> GPGSMSETIIEKYADTDALVTAAGDRLASAITGALAERGKAMIVLTGGGTGIALLKHLRDVASGLDWTNVHVFWGDDRYVPKTDPERNAWQAWEALLEHVNFPLRNMHAMPNSESEYGTDL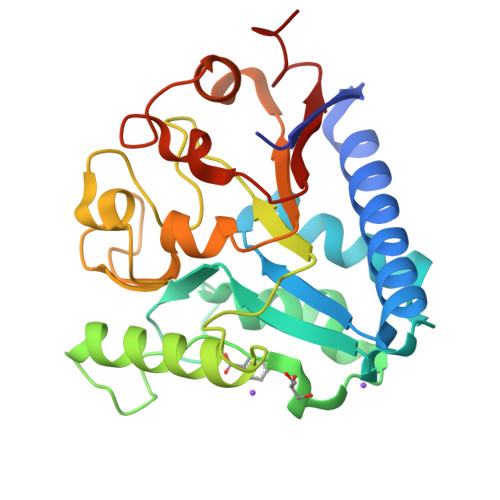DAAALAYEQLLAANAEPGQDCPAFDVHLLGMGGEGHINSLFPHTDAVKETQRLVVAVPDSPKPPPQRITLTLPAIQRSREVWLVVSGEAKADAVAAAVGGADPVDVPAAGAKGIERTVWLLDEAAASQLG> MKNDKKVVVKV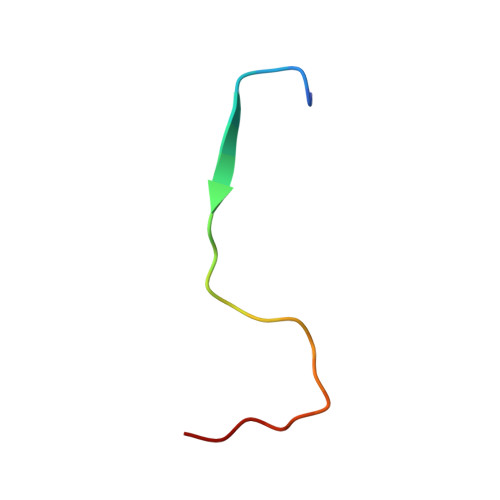KDKEMTCGAFNK> EAPYASLTEIEHLVQSVCKSYRETCQLRL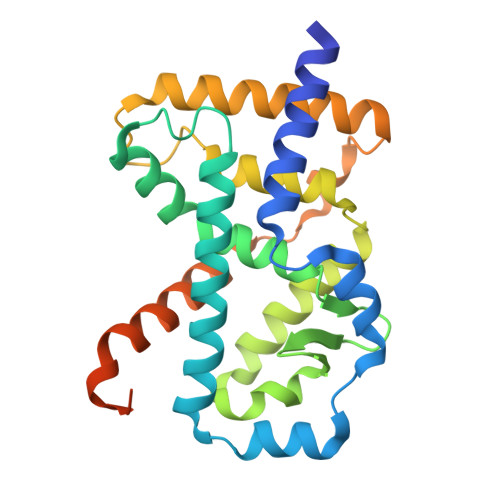EDLLRQRSNIFSREEVTGYQRKSMWEMWERCAHHLTEAIQYVVEFAKRLSGFMELCQNDQIVLLKAGAMEVVLVRMCRAYNADNRTVFFEGKYGGMELFRALGCSELISSIFDFSHSLSALHFSEDEIALYTALVLINAHRPGLQEKRKVEQLQYNLELAFHHHLCKTHRQSILAKLPPAGKLASLCSQHVERLQIFQHLHPIVVQAAFPPLYKELFSTETESPVGLSK>RDHRKIGKQLDLYHMQEEAPGMVFWHNDGWTIFRELEVFVRSKLKEYQYQEVKGPFMMDRVLWEKTGHWDNYKDAMFTTSSENREYCIKPMNCPGHVQIFNQGLKSYRDLPLRMAEFGSCHRNEPSGSLHGLMRVRGFTQDDAHIFCTEEQIRDEVNGCIRLVYDMYSTFGFEKIVVKLSTRPEKRIGSDEMWDRAEADLAVALEENNIPFEYQLGEGAFYGPKIEFTLYDCLDRAWQCGTVQLDFSLPSRLSASYVGEDNERKVPVMIHRAILGSMERFIGILTEEFAGFFPTWLAPVQVVIMNITDSQSEYVNELTQKLSNAGIRVKADLR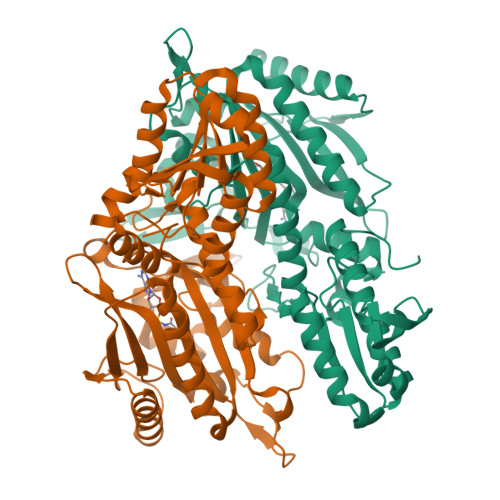NEKIGFKIREHTLRRVPYMLVCGDKEVESGKVAVRTRRGKDLGSMDVNEVIEKLQQEIRSRSLKQLEE[2x]(1S,2S)-1-(2,4-DIAMINOPTERIDIN-6-YL)PROPANE-1,2-DIOL | C9 H12 N6 O2 | 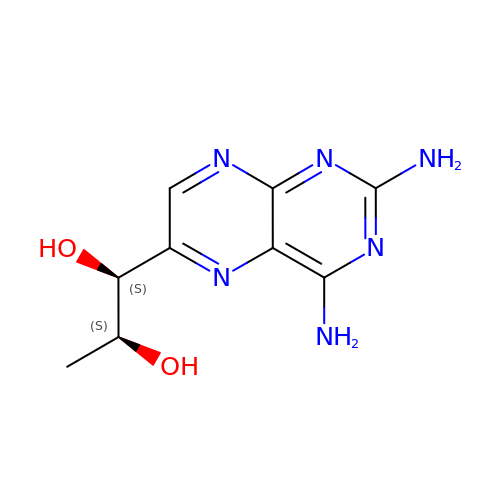ADPRPNXHOYFHIT-BBIVZNJYSA-N>GSEELLDLFNRQVTQEFTASQVYLSASIWFDQNDWEGMAAYMLAHSAEEREHGLGFVDFANKRNIPIELQAVPAPVSCAEWSSPEDVWQSILELEQANTRSLLNLAEAA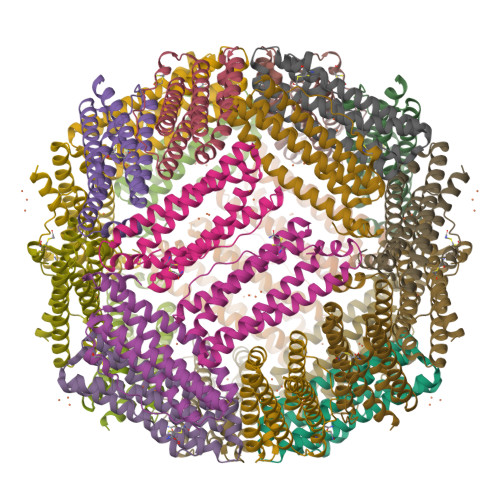STCHDFAVMAFLNPFHLQQVNEEDKIGSILAKVTDENRTPGLLRSLDVVSFLGPCLFRSV[6x]>[2x]MLMIDENPHYKTSIKPNKSYKFGLLTIGSRGDVQPYIALGKGLIKEGHQVVIITHSEFRDFVESHGIQFEEIAGNPVELMSLMVENESMNVKMLREASSKFRGWIDALLQTSWEVCNRRKFDILIESPSAMVGIHITEALQIPYFRAFTMPWTRTRAYPHAFIVPDQKRGGNYNYLTHVLFENVFW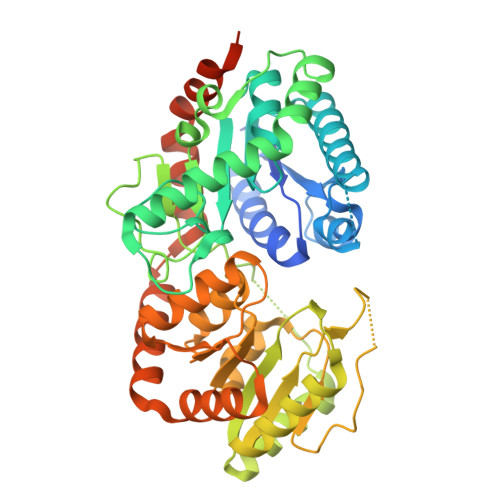KGISGQVNKWRVETLGLGKTNLFLLQQNNVPFLYNVSPTIFPPSIDFSEWVRVTGYWFLDDKSTFKPPAELQEFISEARSKGKKLVYIGFGSIVVSNAKEMTEALVEAVMEADVYCILNKGWSERLGDKAAKKTEVDLPRNILNIGNVPHDWLFPQVDAAVHHGGSGTTGASLRAGLPTVIKPFFGDQFFYAGRVEDIGVGIALKKLNAQTLADALKVATTNKIMKDRAGLIKKKISKEDGIKTAISAIYNELEYARSVTLSRVKTPRKKEENVDATKLTPAETTDEGWTMI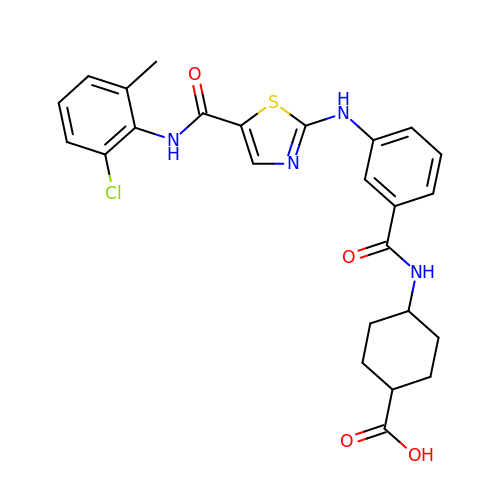4-[[3-[[5-[(2-chloranyl-6-methyl-phenyl)carbamoyl]-1,3-thiazol-2-yl]amino]phenyl]carbonylamino]cyclohexane-1-carboxylic acid | C25 H25 Cl N4 O4 S | AJRURWGSRUYOQL-JCNLHEQBSA-N> AMD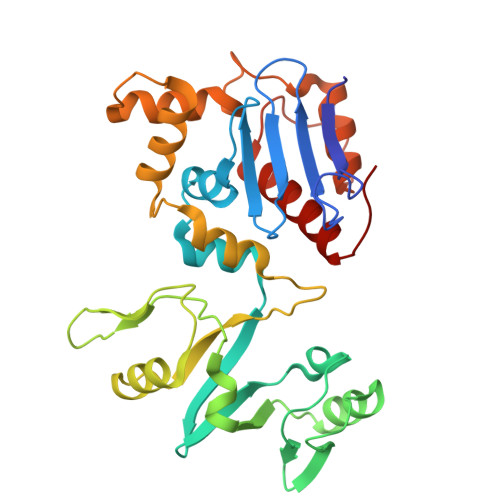SPGVFFDSDKGKTHSSGKVLYNARIIPYRGSWLDFEFDPKDNLFVRIDRRRKLPATIILRALNYTTEQILDLFFEKVIFEIRDNKLQMELVPERLRGETASFDIEANGKVYVEKGRRITARHIRQLEKDDVKLIEVPVEYIAGKVVAKDYIDESTGELICAANMELSLDLLAKLSQSGHKRIETLFTNDLDHGPYISETLRVDPTNDRLSALVEIYRMMRPGEPPTREAAESLFENLFFSEDRYDLSAVGRMKFNRSLLREEIEGSGILSKDDIIDVMKKLIDIRNGKGEVD> PISPIETVPVKLKPGMDGPKVKQWPLTEEKIKALVEICTELEKEGKISKIGPENPYNTPVFAIKKKNSTRWRKLVDFRELNKRTQDFWEVQLGIPHPAGLKKKKSVTVLDVGDAYFSVPLDEDFRKYTAFTIPSINNETPGIRYQYNVLPQGWKGSPAIFQSSMTKILEPFRKQNPDIVIYQYVDDLYVGSDLEIGQHRTKIEELRQHLLRWGLYTPDKKHQKEPPFLWMGYELHPDKWTVQPIVLPEKDSWTVNDIQKLVGKLNWASQIYPGIKVRQLCKLLRGTKALTEVIPLTEEAELELAENREILKEPVHGVYYDPSKDLIAEIQKQGQGQ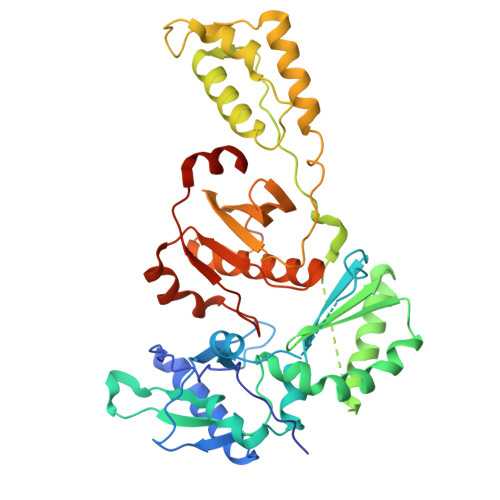WTYQIYQEPFKNLKTGKYARMRGAHTNDVKQLTEAVQKITTESIVIWGKTPKFKLPIQKETWETWWTEYWQATWIPEWEFVNTPPLVKLWYQLEKEPIVGAETF>[2x]MRILLATDGSPQARGAEALAEWLAYKLSAPLTVLFVVDT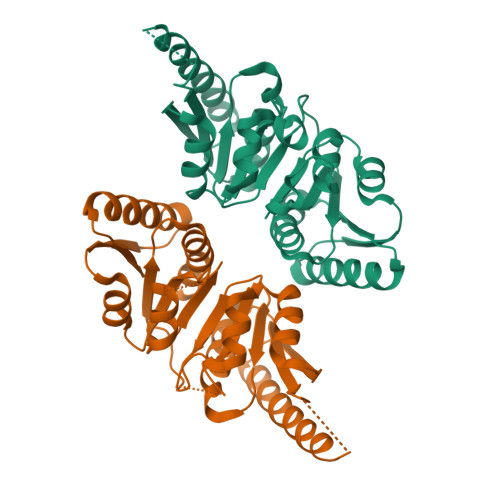RLARIPELLDFGALTVPVPVLRTELERALALRGEAVLERVRQSALAAGVAVEAVLEEGVPHEAILRRARAADLLVLGRSGEAHGDGFGGLGSTADRVLRASPVPVLLAPGEPVELEGALLGYDASESAVRALHALAPLARALGLGVRVVSVHEDPARAEAWALEAEAYLRDHGVEASALVLGGDAADHLLRLQGPGDLLALGAPVRRLVFGSTAERVIRNAQGPVLTAR>[2x]ANPCCSNPCQNRGECMSTGFDQYKCDCTRTGFYGENCTTPEFLTRIKLLLKPTPNTVHYILTHFKGVWNIVNNIPFLRSLIMKYVLTSRSYLIDSPPTYNVHYGYKSWEAFSNLSYYTRALPPVADDCPTPMGVKGNKELPDSKEVLEKVLLRREFIPDPQGSNMMFAFFAQHFTAQFFKTDHKRGPGFTRGLGHGVDLNHIYGETLDRQHKLRLFKDGKLKYQVIGGEVYPPTVKDTQVEMIYPPHIPENLQFAVGQEVFGLVPGLMMYATIWLREHQRVCDILKQEHPEWGDEQLFQTSKLILIGETIKIVIEDYVQHLSGYHFKLKFDPELLFNQQFQYQNRIASEFNTLYHWHPLLPDTFNIEDQ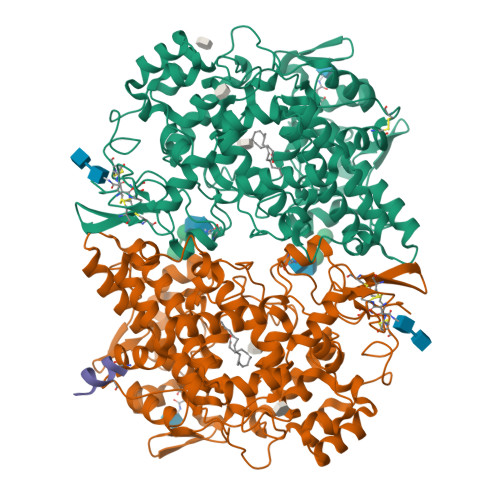EYSFKQFLYNNSILLEHGLTQFVESFTRQIAGRVAGGRNVPIAVQAVAKASIDQSREMKYQSLNEYRKRFSLKPYTSFEELTGEKEMAAELKALYSDIDVMELYPALLVEKPRPDAIFGETMVELGAPFSLKGLMGNPICSPQYWKPSTFGGEVGFKIINTASIQSLICNNVKGCPFTSFNVQ;> TKTATINAS>QMQKEQLNLMPWPQNVVVNDGNFTLTKNFKVNISGNPDSRIFGGVTRFLRRLDGRTGIFFEQGFITKLNEFPNAELQINCTKNGKIGLYEDESYSLDVKANKITINATSDLGALHGLETLLQLLQNDSKKFYFPVSQISDFPRFTWRGLMLDASRHFQPVDVVKRNLDALAAMKMNVFHWHLVDDQGWRIETKKHPKLIELASDGLYYTQEEIRNIVKYADERGILIVPEIDVPGHGSAILTAYPEIGSKVITLTGGTSEKNIQGTAISTYRIERNAGIFSPTLDPSNPKTYKILSELFDEVCPLFPGAYFHIGGDENEGKDWDANPKIQEFKKKHNLKTNHELQTYFTMQLAPMLKKHGKQLMGWEEILTKDLSKEAIVHSWRGPNEGMVAGQSLVDAVKKGYKTVLSNGFYIDLMYPVASHYLNDPMPKGADLSAEEKARILGGEATMWTELATPETFDSRVWPRTAAIAERLWSAENITDVANMRKRLESVSFRLEELGLTHIKNKAVILRNIANNQNIKSVNEFTNVCEPLKGYTRNKGGTEYQMYSPFTLFADACTPDAKDSLAFDEAVSQYLANKSADNKAKVAAFFNKWIAVNKGLVELSANAPLVQPILPLSKKLSDASQELLLVLDNKSTLKTADLKTLIEQCNTKDHADVELSVYESLKKLIA[2x]

No culturable Bacteroidete has yet conclusively been shown to deconstruct cellulose via the actions of a PUL7, but we recently identified and characterized a chitin utilization locus (ChiUL) from the aerobic soil bacterium Flavobacterium johnsoniae. The F. johnsoniae ChiUL consists of 11 genes: two SusC/D-like pairs for oligosaccharide capture and transport, an inner membrane transporter, a two-component sensor/regulator pair, and four enzymes. Here we present the crystal structures of the FjChiB chitinase and the FjGH20 chitobiase, as well as a small-angle X-ray scattering (SAXS) envelope of the novel FjChiA_M domain.

The fourth enzyme, the FjGH20 chitobiase/N-acetylglucosaminidase, was active only on CHOs. Thus, to illuminate these features we pursued structural determination of the FjGH20 by X-ray crystallography and were able to solve the protein structure from diffraction data extending to 1.70 Å resolution. The crystallographic asymmetric unit contained two protein molecules whose interaction gives rise to a buried surface area of ~ 11%, as determined by PISA21. Analysis of the protein in solution by size exclusion chromatography was consistent with a monomer unit being the prominent species (≥ 80%) and thus the dimer observed in the crystal structure is likely not of biological relevance. Each protomer consists of three domains: a central domain (residues 145–502) composed of a (β/α)8 TIM-barrel, an N-terminal domain (residues 1–144) comprising a six-stranded β-sheet and two α-helices where the helices are sandwiched between the β-sheet and the central domain, and a C-terminal domain (residues 504–673) consisting of an eight-helix bundle with two short β-strands. Several of the active site residues shown to be important for substrate binding and catalysis in GH20 members are conserved in FjGH20, including the H-x-G-G-D-E motif where a glutamic acid (Glu317) is proposed to act as a general acid/base in the reaction. The FjGH20 substrate-binding pocket is distinct in one significant way compared to the archetypical GH20 from S. marcescens (SmGH20)20,25 in that FjGH20 lacks the extended loop that is located between β-strand 7 and α-helix 7 in SmGH20. Interestingly, a portion of a loop extending from the FjGH20 helical bundle domain wraps around, and closes off, one side of the active site cleft in the TIM barrel with a tyrosine residue (Tyr538) that projects its sidechain into a position similar to the Trp685 residue in SmGH20. The FjGH20 C-terminal helical bundle is a distinct domain amongst structurally determined GH20 family members.>GPCSNHADSLNNLANIKREQGYIEEATRLYLKALEVFPDFAAAHSNLASVLQQQGKLKEALMHYKEAIRIQPTFADAYSNMGNTLKELQDVSGALQCYTRAIQINPAFADAHSNLASIHKDSGNIPEAIQSYRTALKLKPDFPDAYCNLAHCLQIVCDWTDYDIRMKKLVSIVTEQLEKNRLPSVHPHHSMLYPLTHDCRKAIAARHANLCLEKVHVLHKKPYNFLKKLPTKGRLRIGYLSSDFGNHPTSHLMQSVPGLHDRSKVEIFCYALSPDDGTTFRHKISRESENFVDLSQIPCNGKAADKIFNDGIHILVNMNGYTKGARNEIFALRPAPIQVMWLGYPGTSGASFMDYIITDSVTSPLELAYQYSEKLSYMPHTYFIGDHKQMFPHLKERIIVCDKQQSSVVDNVTVINATDLSPLVENTDVKEIKEVVNAQKPVEITHKVAELPNTTQIVSMIATGQVQTSLNGVVVQNGLATTQTNNKAATGEEVPQNIVITTRRQYMLPDDAVVYCNFNQLYMIDPQTLESWVEILKNVPKSVLWLLRFPAVGEQNIKKTVSDFGISPDRVIFSNVAAKEEHVRRGQLADICLDTPLCNGHTTSMDVLWTGTPVVTLPGETLASRVAASQLATLGCPELIARTREEYQNIAIRLGTKKEYLKALRAKVWKARVESPLFDCSQYAKGLEKLFLRMWEKYENGELPDHISAV[3x]

The enzyme that catalyses the addition of a single GlcNAc onto serine/threonine residues on intracellular proteins is O-GlcNAc transferase (OGT). OGT is highly conserved in metazoa, consisting of a C-terminal glycosyltransferase domain and N-terminal tetratricopeptide repeats (TPRs). In Drosophila, ogt is known as super sex combs (sxc), mutants of which do not develop beyond the pharate adult stage. sxc belongs to the Polycomb group (PcG) genes that play key roles in developmental regulation, stem-cell maintenance and genomic imprinting. Sequence similarity between hOGT and DmOGT is high, with 90% and approximately 80% sequence identity in the TPR region and the catalytic domain, respectively.

To determine how differences in sequence influence the overall structure of DmOGT and to provide a template for structure-guided mutagenesis, an N-terminally truncated construct starting at amino acid 353 in TPR 10 (Δ1–352) carrying a mutation (K872M) of a key catalytic lysine was expressed in Escherichia coli and crystallized in complex with the inhibitor/substrate analogue UDP-5S-GlcNAc. The structure was solved by molecular replacement and refined against 2.7 Å synchrotron diffraction data, yielding clear electron density for UDP-5S-GlcNAc. Crystals belonged to space group P32 and contained 3 molecules per asymmetric unit. It appears that DmOGT adopts the canonical OGT fold with the bilobal arrangement of two Rossmann-like domains characteristic of the GT-B superfamily of glycosyltransferases, as well as the additional TPR-like helices (535–566) in the N-terminal of the catalytic domain, which lead into the TPR domain. As a result, the TPRs are in close association with the glycosyltransferase domain and the catalytic site is aligned with the channel along the main axis of the TPR superhelix. The catalytic site residues (H537, H596, Y871, K872, K928, H932, R935, H951, D955) that are found to interact with UDP-GlcNAc and the acceptor peptides in hOGT are conserved and similarly positioned in DmOGT, suggesting a similar catalytic mechanism involving the same UDP-GlcNAc and acceptor peptide binding modes. The intervening domain, a 100-amino acid insertion between the two Rossmann-like folds of the catalytic domain, is the site of lowest sequence conservation and highest degree of flexibility in the structures of both hOGT and DmOGT. Three short loops were disordered, but the overall domain architecture mirrors that of the hOGT intervening domain. Activity of the Δ1–352 DmOGT is inhibited by UDP-5S-GlcNAc with an inhibition constant (Ki) of 36.2 µM, comparable with the Ki of Δ1–313 hOGT at 13.6 µM. The absence of a similar positively charged patch on the surface of DmOGT further weakens the hypothesis that PIP3 binding in general could regulate the subcellular localization of OGT.>KLANVVILATGGTIAGAGASAANSATYQAAKVGVDKLIAGVPELADLANVRGEQVMQIASESITNDDLLKLGKRVAELADSNDVDGIVITHGTDTLEETAYFLNLVQKTDKPIVVVGSMRPGTAMSA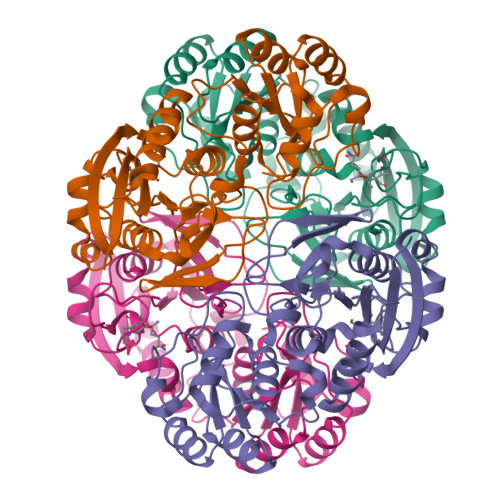DGMLNLYNAVAVASNKDSRGKGVLVTMNDEIQSGRDVSKSINIKTEAFKSAWGPLGMVVEGKSYWFRLPAKRHTVNSEFDIKQISSLPQVDIAYSYGNVTDTAYKALAQNGAKALIHAGTGNGSVSSRVVPALQQLRKNGTQIIRSSHVNQGGFVLRNAEQPDDKNDWVVAHDLNPEKARILAMVAMTKTQDSKELQRIFWEY[2x]> MKKIEAIIKPFKLDEVKDALVEIGIGGMTVTEVKGFGQQKGHTEIYRGTEYVIDFLPKV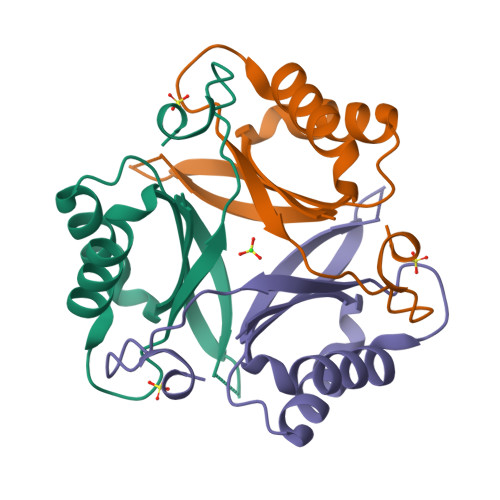KIEVVVRDEDVEKVVETIVKTAQTGRVGDGKIFIIPVEDVIRIRTGERGEQAI>MTGDHIKVIYFNGRGRAESIQMTLVAAGVNYEDERISFQDWPKIKPTIPGGRLPAVKITDNHGHVKWMVESLAIARYMAKKHHMMGGTEEEYYNVEKLIGQAEDLEHEYYKTLMKPEEEKQKIIKEILNGKVPVLLDIICESLKASTGKLAVGDKV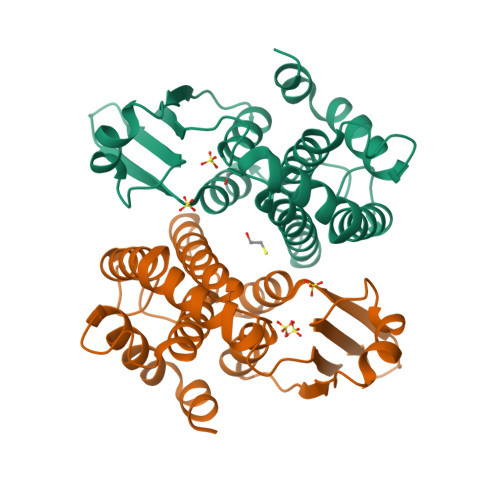TLADLVLIAVIDHVTDLDKEFLTGKYPEIHKHRENLLASSPRLAKYLSDRAATPF[2x]> ISEFMSDITVTNWAGNITYTAKELLRPHSLDALRALVADSARVRVLGSGHSFNEIAEPGDGGVLLSLAGLPSVVDVDTAARTVRVGGGVRYAELARVVHARGLALPNMASLPHISVAGSVATGTHGSGVGNGSLASVVREVELVTADGSTVVIARGDERFGGAVTSLGALGVVTSLTLDLEPAYEMEQHVFTELPLAGLDPATFETVMAAAYSVSLFTDWRAPGFRQVWLKRRTDRPLDGFPYAAPAAEKMHPVPGMPAVNCTEQFGVPGPWHERLPHFRAEFTPSSGAELQSEYLMPREHALAALHAMDAIRETLAPVLQT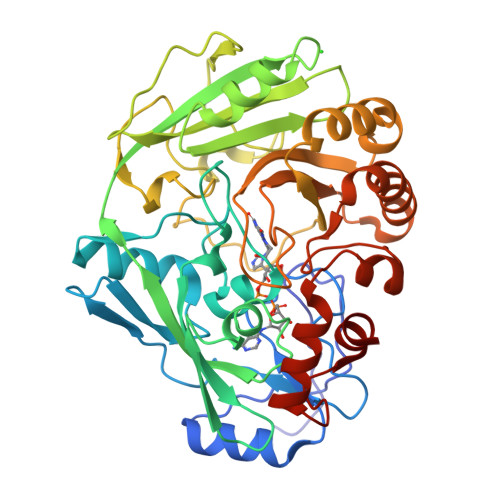CEIRTVAADAQWLSPAYGRDTVAAHFTWVEDTAAVLPVVRRLEEALVPFAARPHWGKVFTVPAGELRALYPRLADFGALAGALDPAGKFTNAFVRGVLAG>[4x]MGSDKIHHHHHHMMERLIGSTPIVRLDSIDSRIFLKLEKNNPGGSVKDRPALFMILDAEKRGLLKNGIVEPTSGNMGIAIAMIGAKRGHRVILTMPETMSVERRKVLKMLGAELVLTPGELGMKGAVEKALEISRETGAHMLNQFENPYNVYSHQFTTGPEILKQMDYQIDAFVAGVGTGGTISGVGRVLKGFFGNGVKIVAVEPAK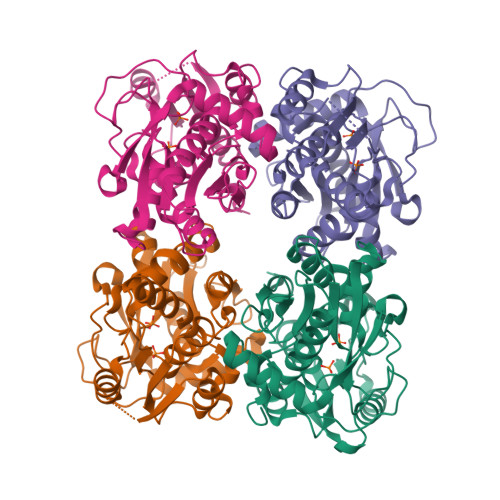SPVLSGGQPGKHAIQGIGAGFVPKILDRSVIDEVITVEDEEAYEMARYLAKKEGLLVGISSGANVAAALKVAQKLGPDARVVTVAPDHAERYLSIL>MPNSEPASLLELFNSIATQGELVRSLKAGNASKDEIDSAVKMLVSLKMSYKAAAGEDYKADCPPGNPAPTSNHGPDATEAEEDFVDPWTVQTSSAKGIDYDKLIVRFGSSKIDKELINRIERATGQRPHHFLRRGIFFSHRDMNQVLDAYENKKPFYLYTGRGPSSEAMHVGHLIPFIFTKWLQDVFNVPLVIQMTDDEKYLWKDLTLDQAYSYAVENAKDIIACGFDINKTFIFSDLDYMGMSSGFYKNVVKIQKHVTFNQVKGIFGFTDS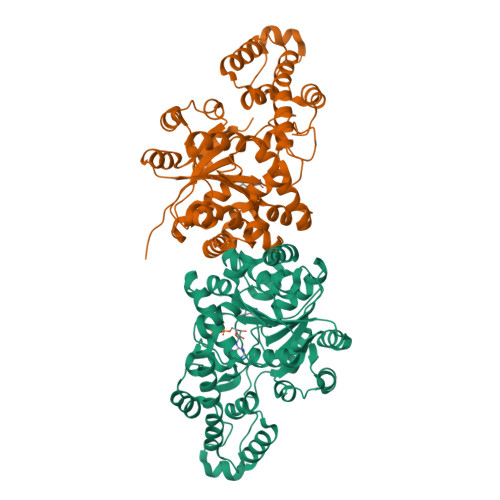DCIGKISFPAIQAAPSFSNSFPQIFRDRTDIQCLIPCAIDQDPYFRMTRDVAPRIGYPKPALLHSTFFPALQGAQTKMSASDPNSSIFLTDTAKQIKTKVNKHAFSGGRDTIEEHRQFGGNCDVDVSFMYLTFFLEDDDKLEQIRKDYTSGAMLTGELKKALIEVLQPLIAEHQARRKEVTDEIVKEFMTPRKLSFDFQHHHHHH[2x]>MSSYLDDLRIDLAASPASGGSASIAVGSFNIPYEVTRRLKGVGADADTTLTSCASWTQLQKLYEQYGDEPIKKHFETDSERGQRYSVKVSLGSKDENFLFLDYSKSHINDEIKCALLRLAEERGIRQFVQSVFRGERVNTTENRPVLHIALRNRSNRPIYVDGKDVMPAVNKVLDQMRSFSEKVRTGEWKGHTGKAIRHVVNIGIGGSDLGPVMATEALKPFSQRDLSLHFVSNVDGTHIAEVLKSIDIEATLFIVASKTFTTQETITNALSARRALLDYLRSRGIDEKGSVAKHFVALSTNNQKVKEFGIDEENMFQFWDWVGGRYSMWSAIGLPIMISIGYENFVELLTGAHVIDEHFANAPPEQNVPLLLALVGVWYIN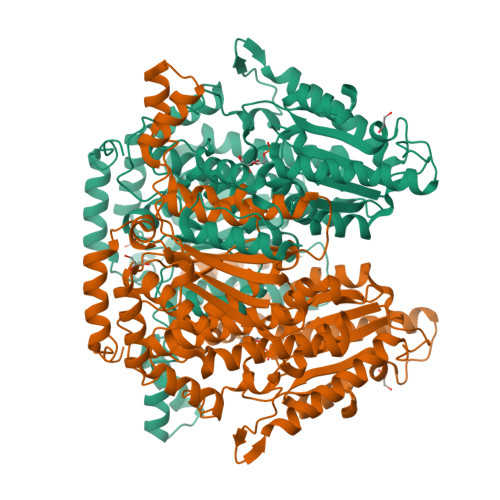FFGAVTHAILPYDQYLWRLPAYLQQLDMESNGKYVTRSGKTVSTLTGPIIFGEAGTNGQHAFYQLIHQGTNLIPCDFIGAIQSQNKIGDHHKIFMSNFFAQTEALMIGKSPSEVRRELEAAGERSAEKINALLPHKTFIGGRPSNTLLIKSLTPRALGAIIAMYEHKVLVQGAIWGIDSYDQWGVELGKVLAKSILPQLRPGMRVNNHDSSTNGLINMFNELSHLHHHHHH[3x]> 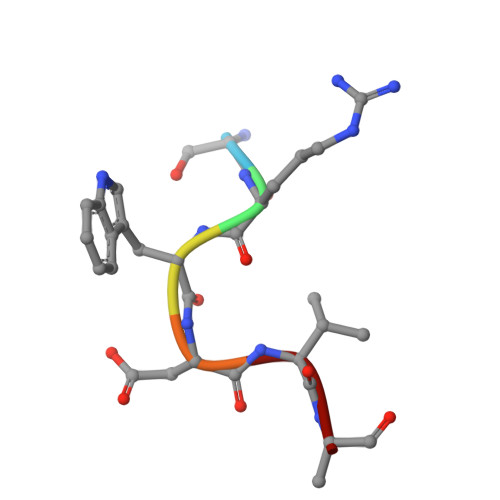SRWDVK> GEITSVSTACQQLEVFSRVLRTSLATILDGGEENLEKNLPEFAKMVCHGEHTYLFAQAMMSVLAQEEQGGSAVRRIAQEVQRFAQEKGHDASQITLALGTAASYPRACQALGAMLSKGALNPADITVLFKMFTSMDPPPVELIRVPAFLDLFMQSLFKPGARINQDHKH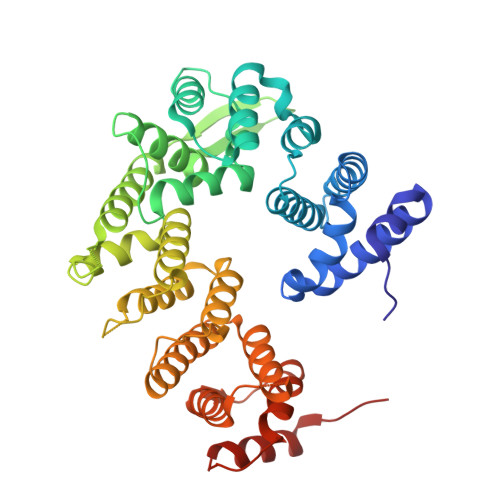KYIHILAYAASVVETWKKNKRVSINKDELKSTSKAVETVHNLCCNENKGASELVAELSTLYQCIRFPVVAMGVLKWVDWTVSEPRYFQLQTDHTPVHLALLDEISTCHQLLHPQVLQLLVKLFETEHSALDVMEQLELKKTLLDRMVHLLSRGYVLPVVSYIRKCLEKLDTDISLIRYFVTEVLDVIAPPYTSDFVQLFLPILENDSIAGTIKTEGEHDPVTEFIAHCKSNFIMVN3-(INDOL-3-YL) LACTATE | C11 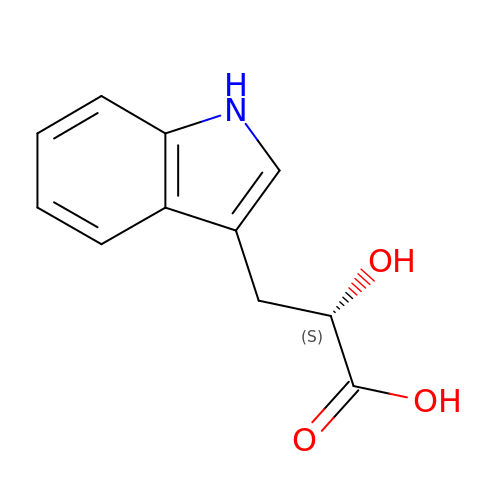H11 N O3 | XGILAAMKEQUXLS-JTQLQIEISA-N>[6x]MLVVGSELQSDAQQLSAEAPRHGELQYLRQVEHILRCGFKKEDRTGTGTLSVFGMQARYSLRDEFPLLTTKRVFWKGVLEELLWFIKGSTNAKELSSKGVRIWDANGSRDFL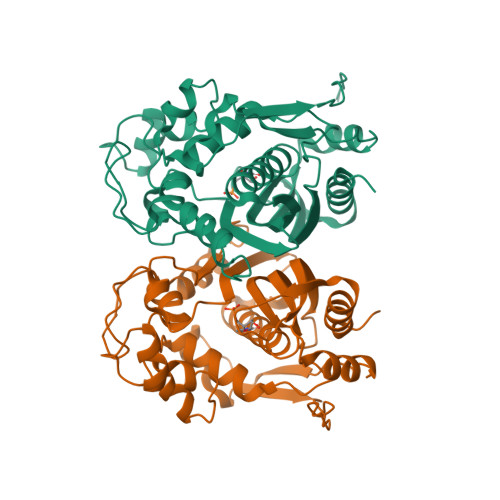DSLGFSARQEGDLGPVYGFQWRHFGAEYKDMDSDYSGQGVDQLQKVIDTIKTNPDDRRIIMCAWNPKDLPLMALPPCHALCQFYVVNGELSCQLYQRSGDMGLGVPFNIASYALLTYMIAHITGLQPGDFVHTLGDAHIYLNHIEPLKIQLQREPRPFPKLKILRKVETIDDFKVEDFQIEGYNPHPTIKMEMAV> SELIVNVINGPSLGRLGRREPAVYGGTTHDELVALIEREAAELGLKAVVRQSDSEAQL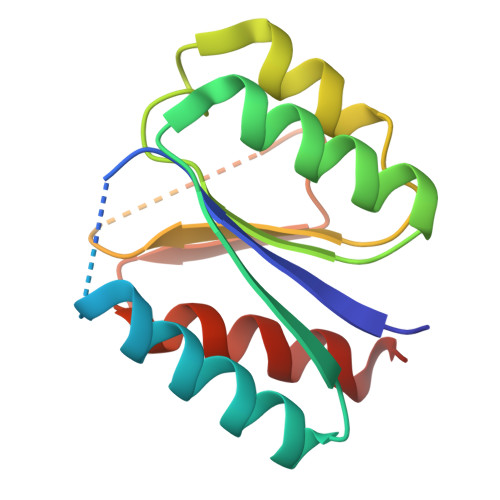LDWIHQAADAAEPVILNAGGLTHTSVALRDACAELSAPLIEVHISNVHAREEFRRHSYLSPIATGVIVGLGIQGYLLALRYLAEHVGT8-[4-(2-azanylethyl)pyrazol-1-yl]-3H-pyrido[3,4-d]pyrimidin-4-one 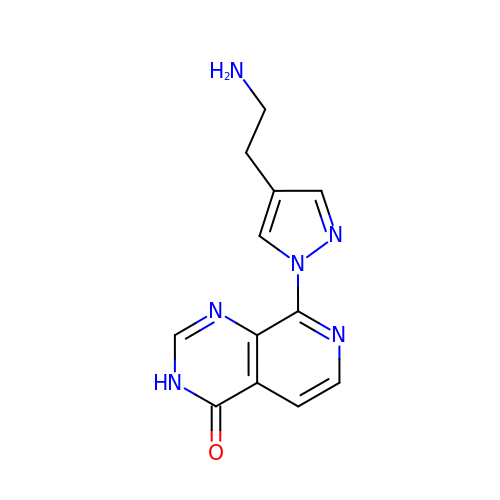| C12 H12 N6 O | YNSLRVQPGFUMPO-UHFFFAOYSA-N> MLSRKGIIPEEYVLTRLAEDPAKPRYRARQRRARFVSKKGNCNVAHKNIREQGRFLQDVFTTLVDLKWPHTLLIFTMSFLCSWLLFAMAWWLIAFAHGDLAPSEGTAEPCVTSIHSFSSAFLFSIEVQVTIGFGGRMVTEECPLAILILIVQNIVGLMINAIMLGSIFMKTAQAHRRAETLIFSKHAVIALRHGRLCFMLRVGDLRKSMIISATIHMQVVRKTTSPEGEVVPLHQVDIPMENGVGGNSIFLVAPLIIYHVIDANSPLYDLAPSDLHHHQDLEIIVILEGVVETTGITTQARTSYLADEILWGQRFVPIVAEEDGRYSVDYSKFDNTVKVPTPLCTARQLDEDHSLLEALTLASARGPLRKRSVPMAK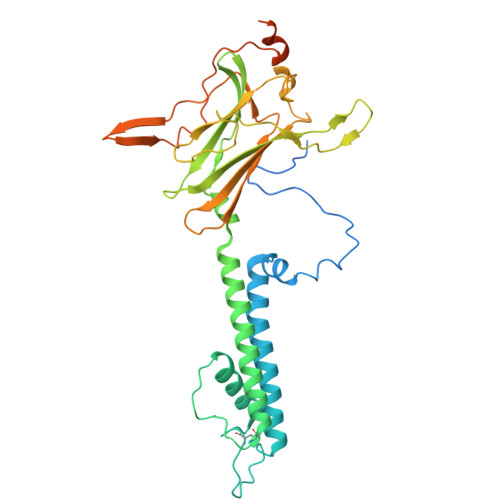AKPKFSISPDSLS>MLNL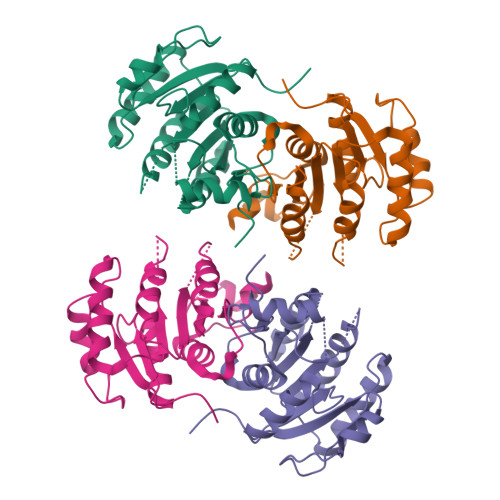ENKTYVIMGIANKRSIAFGVAKVLDQLGAKLVFTYRKERSRKELEKLLEQLNQPEAHLYQIDVQSDEEVINGFEQIGKDVGNIDGVYHSIAFANMEDLRGRFSETSREGFLLAQDISSYSLTIVAHEAKKLMPEGGSIVATTYLGGEFAVQNYNVMGVAKASLEANVKYLALDLGPDNIRVNAISAGPIRTLSAKGVGGFNTILKEIEERAPLKRNVDQVEVGKTAAYLLSDLSSGVTGENIHVDSGFHAIK[2x]>MAKEVVEVLVTGGRATAGPPLGPAIGPLGVNVMQVVKEINEKTKDYEGMQVPVKVIVDTETRKFEIEVGIPPTTALIKKELGIETAAHEPRHEVVGNLTLEQVIKIAKMKKDAMLSYTLKNAVKEVLGTCG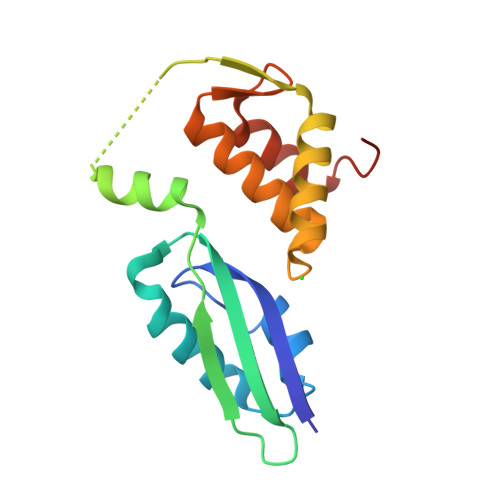SMGVTVEGKDPKEVQKEIDAGVYDEYFKEE[2x]> GSTMHTDGDKAFVDFLSDEIKEERKIQKHKTLPKMSGGWELELNGTEAKLVRKVAGEKITVTFNINNSGGSTPNFVVEVIKNDDGKKALVLDCHYGDIFSIREVSFQSTGESEWKDTNYTLNTDSLDWALYDHLMDFLADRGVDNTFADELVELSTALEHQEYITFLEDLKSFVKSQ

gC1qR/C1qBP/HABP-1 is a multicompartmental and multifunctional protein that undergoes spatiotemporal changes in its distribution in response to various cellular and systemic stimuli. Although it normally functions within the cell and plays an essential role in mitochondrial biogenesis by virtue of its mRNA binding activity (2), gC1qR exposed at the cellular surface serves as a route to gain cellular entry for numerous pathogens as well as acting as an inflammatory trigger in a number of other diseases including vascular disorders and various cancers [Reviewed in (1)]. Chief among these is oligomerization of the gC1qR monomer into a toroidal, ring-like trimer. Although these loops are disordered in the gC1qR crystal structure, they themselves are rich in acidic residues and project outward from the negatively charged face of the gC1qR trimer.

To address these limitations, we used the existing crystal structure of mature gC1qR to design individual deletion mutants of Loop 1 (i.e. gC1qR-D1) and Loop 2 (i.e. gC1qR-D2) wherein the entire acidic loop was replaced with either two or one glycine residue(s), respectively. In addition to this, we designed a double deletion mutant that simultaneously removed both Loop 1 and Loop 2 (i.e. gC1qR-DD) using the same strategy described above. We collected X-ray diffraction data to 2.2 Å limiting resolution and solved the structure of gC1qR-DD by molecular replacement using the published structure of the wild-type gC1qR monomer as a search model. The asymmetric unit of the crystal contained a single copy of the gC1qR-DD polypeptide from residues 76-247, aside from two discontinuities in regions connecting α1-β1 (i.e. residues 98-100) and β3-β4 (i.e. residues 138-141) due to weak electron density in those areas. Although the final model contained only a single copy of the gC1qR-DD polypeptide, the structure of the gC1qR-DD trimer that exists in solution could be reconstructed by applying crystallographic symmetry. The structure of the gC1qR-DD trimer superimposes well upon on that of wild-type gC1qR, as 140 of the 165 Cα positions align with a root mean square deviation of 0.544 Å. As expected, the primary areas of structural divergence are found in the areas corresponding to the loop deletions. We found that gC1qR-DD behaved as a trimer in solution and this arrangement was likewise visible in its crystal structure. Intriguingly, we found that surface-captured gC1qR-DD bound with low-nanomolar apparent affinity to both FXII and FXIIa. Thus, while gC1qR-DD clearly bound tighly to both FXII and FXIIa, comparison of this mutant to wild-type gC1qR strongly suggested that interactions of these ligands with gC1qR are mechanistically complex and likely to involve multiple contact sites from each binding partner.>[2x]MTDTIFDYVIVGGGTAGSVLANRLSARPENRVLLIEAGIDTPENNIPPEIHDGLRPWLPRLSGDKFFWPNLTIHRAAEHPGITREPQFYEQGRLLGGGSSVNMVVSNRGLPRDYDEWQALGADGWDWQGVLPYF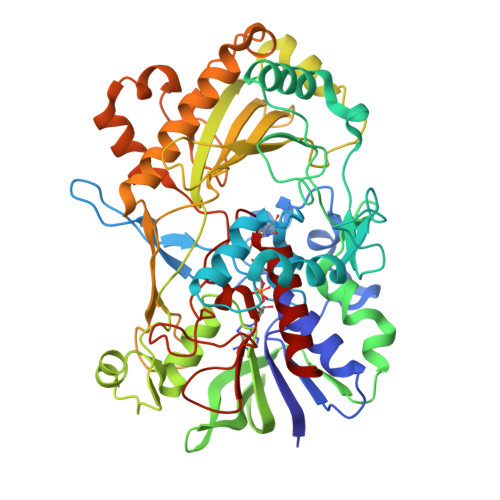IKTERDADYGDDPLHGNAGPIPIGRVDSRHWSDFTVAATQALEAAGLPNIHDQNARFDDGYFPPAFTLKGEERFSAARGYLDASVRVRPNLSLWTESRVLKLLTTGNAITGVSVLRGRETLQVQAREVILTAGALQSPAILLRTGIGPAADLHALGIPVLADRPGVGRNLWEHSSIGVVAPLTEQARADASTGKAGSRHQLGIRASSGVDPATPSDLFLHIGADPVSGLASAVFWVNKPSSTGWLKLKDADPFSYPDVDFNLLSDPRDLGRLKAGLRLITHYFAAPSLAKYGLALALSRFAAPQPGGPLLNDLLQDEAALERYLRTNVGGVWHASGTARIGRADDSQAVVDKAGRVYGVTGLRVADASIMPTVPTANTNLPTLMLAEKIADAILTQA2-phenoxy-5-propyl-phenol | C15 H16 O2 | 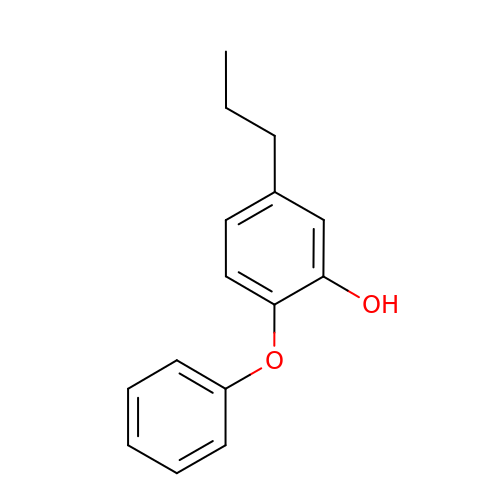JOZACDNAOCTHDN-UHFFFAOYSA-N> GMQEHYQPAAIEPAAQKKWDDARISNVSEDASKPKYYCLSMFPYPSGKLHMGHVRNYTIGDVLSRFKLLNGFNVMQPMGWDAFGMPAENAAMKNNVAPAAWTYDNIEYMKTQLKSLGFAVDWEREVATCKPEYYRWEQWLFTKLFEKGIVYRKNGTVNWDPVDQTVLANEQVIDGRGWRSGALIEKREIPMYYFKITDYAEELLNDLDKLEHWPEQVKTMQRNWIGKSRGMTVRFAVSDDSKQGLEGDYAKFLQVYTTRPDTLMGATYVAVAAEHPLATAAAADKPELQAFIAECKAGSVAEADMATMEKKGVPTGRYVVNPLNGDKLEVWIANYVLWGYGDGAVMAVPAHDERDFEFAAKYNLPKKQVIAVGDNAFDANRWQEWYGDKENGVLVNSGDLDGLDFQTAFDAVAAKLQSQGAGEPKTQYRLRDWGISRQRYWGCPIPIVHCEKCGNVPVPADQLPVVLPENVVPDGMGSPLAKMPEFYETSCPCCGGAAKRETDTMDTFIESSWYFFRYMSPKFSDGMVSAESAKYWGAVDQYIGGIEHAILHLLYARFFTKLMRDEGLVNVDEPFERLLTQGMVVCETYYRENDKGGKDWINPADVELTFDDKGRPVSAVLKADGLPVVISGTEKMSKSKNNGVDPQELINAYGADTARLFMMFAAPPEQSLEWSDSGVEGAHRFLRRLWRTVYEYLKQGGAVKAFAGNQDGLSKELKDLRHKLHSTTAKVSDDYGRRQQFNTAIAAVMELLNQYDKTDTGSEQGRAVAQEVLEAAVRLLWPIVPHICETLWSELNGAKLWEAGWPTVDEAALVKSEIEVMVQVNGKLRGKITVAADASKADLEAAALANEGAVKFMEGKPAKKIIVVPGRLVNIVV

To correctly aminoacylate tRNALeu, leucyl-tRNA synthetase (LeuRS) catalyzes three reactions: activation of leucine by ATP to form leucyl-adenylate (Leu-AMP), transfer of this amino acid to tRNALeu and post-transfer editing of any mischarged product. Mechanistically similar to other adenylate-forming enzymes, the class Ia aminoacyl-tRNA synthetase (aaRS) LeuRS charges tRNALeu isoacceptors, which are essential substrates for protein translation. We have solved crystal structures for all enzymatic states of Neisseria gonorrhoeae LeuRS during Leu-AMP formation.

To capture the different enzymatic states of the first catalytic step of LeuRS, crystals of the N. gonorrhoeae apoenzyme were soaked with Leu, ATP, ATP and l-leucinol, ATP and Leu. As has been previously recognized, the active site of NgLeuRS is large (approximately 758 Å3 in the apo form), which is necessary for association of the various substrates. In the apo state, the synthetic site of NgLeuRS is fully open allowing the entry of all substrates. Comparison of the NgLeuRS apo structure to that of the NgLeuRS·ATP·leucinol ternary complex shows that the CP1 hairpin (residues 147–194) together with a structurally associated α-helix (residues 84–93) rotates 31° toward the active site pushing the editing domain (residues 225–427) 29° away from the same region. Intriguingly, careful examination of the different X-ray structures shows the presence of a peptide-plane flip between L550 and H551 in the NgLeuRS·ATP·leucinol complex, that is absent in the apo and the intermediate bound structures.>[2x]LVSSPTSSGLYVVHIAAEMAPVAKVGGLGDVVAGLGKALQRKGHLVEIILPKYDCMQYDRVRDLRALDTVVESYFDGKLYKNKIWIGTVEGLPVHFIEPQHPSKFFWRGQFYGEQDDFRRFSYFSRAALELLLQSGKKPDIIHCHDWQTAFVAPLYWDLYAPKGLDSARICFTCHNFEYQGTASASELGSCGLDVNQLNRPDRMQDHSSGDRVNPVKGAIIFSNIVTTVSPTYAQEVRTAEGGKGLHSTLNFHSKKFIGILNGIDTDSWNPATDPFLKAQFNAKDLQGKEENKHALRKQLGLSSAESRRPLVGCITRLVPQKGVHLIRHAIYRTLELGGQFVLLGSSPVPHIQREFEGIEQQFKSHDHVRLLLKYDEALSHTIYAASDLFIIPSIFEPCGLTQMIAMRYGSIPIARKTGGLNDSVFDIDDDTIPTQFQNGFTFQTADEQGFNYALERAFNHYKKDEEKWMRLVEKVMSIDFSWGSSATQYEELYTRSVSRARAVPNRT

Starch Synthases (SSs) transfer glucose from ADP-Glc donor to elongate pre-existing glucose chains via α-1,4-linkages. SSs are retaining glycosyltransferases classified within the GT5 family in the Carbohydrate Active Enzyme (CAZy) database. Here we present three new crystal structures of SSs of different families and origins: the crystal structure of the catalytic domain of SSIV from Arabidopsis thaliana (AtSSIV), of GBSS from Cyanobacterium sp. CLg1 (CLg1GBSS) and of GBSSI from the glaucophyte Cyanophora paradoxa (CpGBSSI). In all cases, they are in the closed conformation forming ternary complexes with ADP in the donor site and the inhibitor acarbose occupying the donor glucose and glucose acceptor sites that approximates the active site at the time of the reaction.

The ADP binding mode in the AtSSIV structure will be described to serve as a reference for the other structures. AtSSIV binds ADP through an extensive network of interactions, depicted in Figure 2. While the adenine is bound exclusively to the C-terminal domain of SSIV, the rest of the molecule also interacts with the N-terminal domain. ADP binding occurs through a large number of close interactions and hydrogen bonds, with most of all possible interactions utilized in the case of AtSSIV. Interestingly, the entire set of interactions involving ADP binding to AtSSIV is present in the EcoGS structure, including mediating waters with one exception, the interaction of O2 with Tyr393. Only minor differences are found in the way acarbose is bound in the AtSSIV structure and only these will be mentioned here. The third hexose, here stacked between two tyrosines, has its O6 oriented differently since the threonine bound to it in CLg1GBSS is substituted in AtSSIV by a valine which cannot make side chain hydrogen bonds. Lastly, the reducing glucose is missing the interaction with an aspartate described for CLg1GBSS, as AtSSIV is missing an extra loop present in that region in CLg1GBSS. One new surface binding site for sugars is identified in the AtSSIV structure. Trp172 and Phe237 form an extended and slightly curved aliphatic patch in the surface of the protein, far away from the active site. Fitting of a whole acarbose was unstable and a maltose was modeled there as a generic α-glucan, but the high B factors result in a relatively feature-less density where it is impossible to ascertain the correct geometry of the bound sugars.> GPRLSRLLSYAG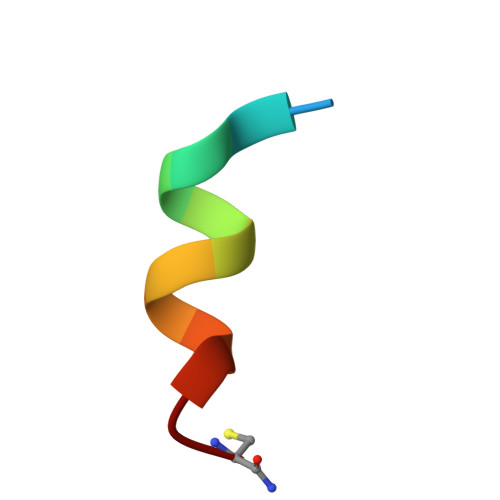C> TVPSSDITNFNEIFYVEPQYIAQAIRLTNTFQGAIDPLTLNFNFEKALQIANGLPNAGVTGTINQSVIHQTIEVSVMISQIKEIIRSVLGLVINSANFWNSVV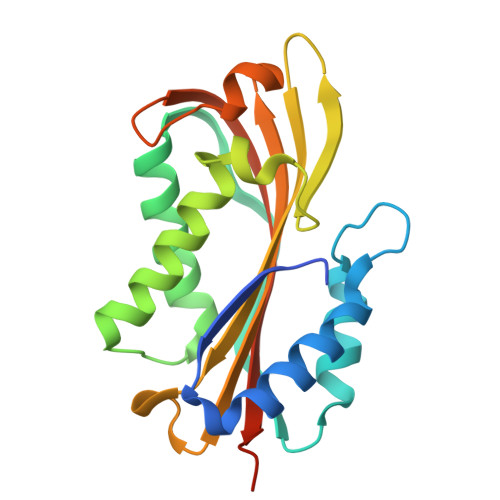SAITNTFTNLEPQVDENWIVWRNLSATQTSYFYKILFSIQNEDTGRFMAILPIAFEITVDVQKQQLLFITIKDSARYEVKMKALTVVQALDSYNAPIIDVF N~6~-[(1Z)-ethanimidoyl]-L-lysine 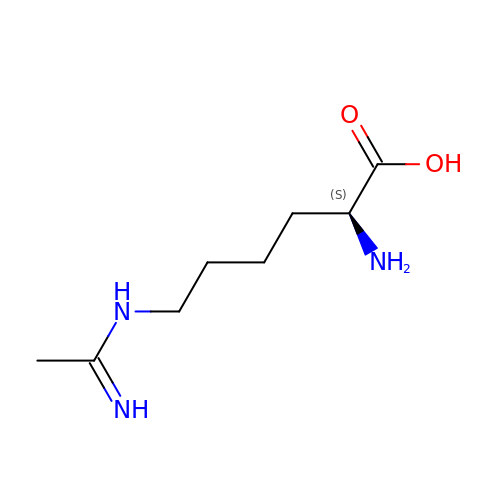| C8 H17 N3 O2 | ONYFNWIHJBLQKE-ZETCQYMHSA-N>MTALNVLIYPDDHLKVVCEPVTEVNDAIRKIVDDMFDTMYQEKGIGLAAPQVDILQRIITIDVEGDKQNQFVLINPEILASEGETGIEEGCLSIPGFRALVPRKEKVTVRALDRDGKEFTLDADGLLAICIQ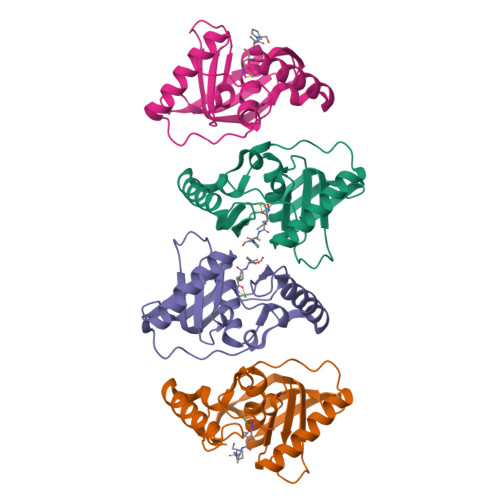HEIDHLNGILFVDYLSPLKRQRIKEKLIKYKKQIAKS[4x]>MIVIPMAGMSSRFFKAGYTQPKYMLEAHGQTLFEHSVNSFAAYFASTPFLFIVRNVYDTAVFVREKATQLGIKQFYIAELHTETRGQAETVTLGLEELAKQGVDYQGSITVFNIDTFRPNFVFPDISQHSDGYLEVFQGGGDNWSFAKPEHAGSTKVIQTAEKNPISDLCSTGLYHFNRKEDYLEAYREYVARPSQEWERGELYIAPLYNELIQKGLNIHYHLIARHEVI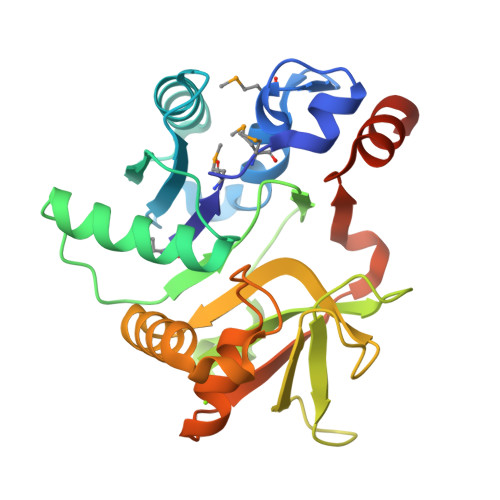FCGVPDEYTDFLRQPQPLEHHHHHH[2x]>MNLIPTVIETTNRGERAYDIYSRLLKDRIIMLGSQIDDNVANSIVSQLLFLQAQDSEKDIYLYINSPGGSVTAGFAIYDTIQHIKPDVQTICIGMAASMGSFLLAAGAKGKRFALPNAEVMIHQPLGGAQGQATEIEIAANHILKTREKLNRILSERTGQSIEKIQKDTDRDNFLTAE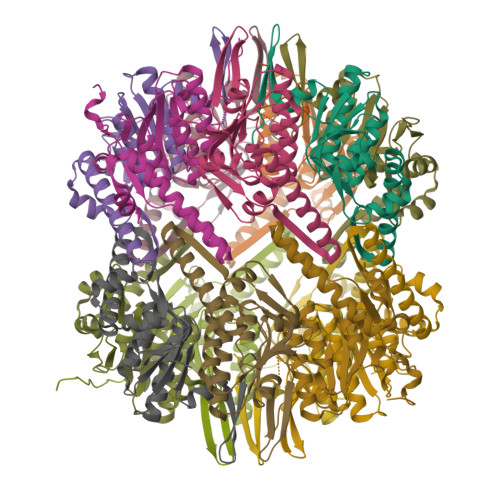EAKEYGLIDEVMVPETKWSHPQFEK[14x]>GMTFRDTSAIASWHAHVYFDASSRDAAWTLREQIEAHWSGKLQLGRFHERPVGPHPMWSYQLAFTQEQFADLVGWLTLNHGALDIFLHP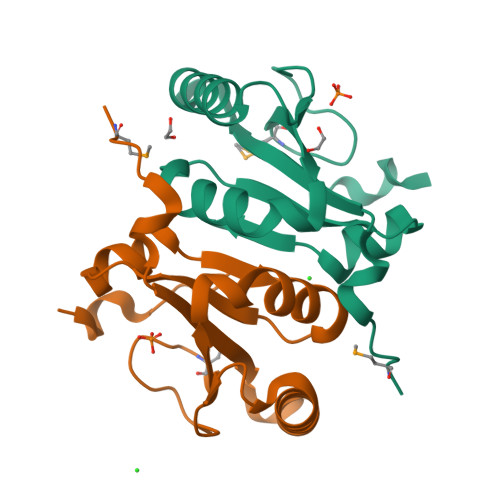NTGDALRDHRDAAVWIGHSHELVLSALN[4x]2-bromanyl-3-phenyl-1~{H}-pyrrolo[3,4-g]indol-8-one | C16 H9 Br N2 O | 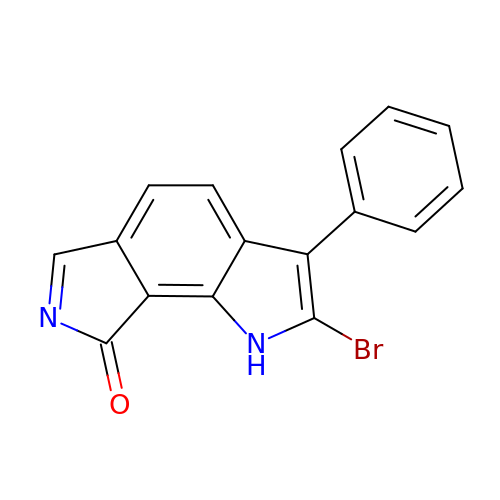VKVBXHZFKDKMDA-UHFFFAOYSA-N> MKKSLGARTLAYPTPLFLVGTYDRDSRPNIMAAAWAGICCSQPPSIAVSLRKATYTYRSITERGAFTISIPSRAYVRHADYAGIYSGENEDKFASLGLTPVPGEHVDAPYVGEFPMAIELKLIHQIEIGLHTQFIGEIMD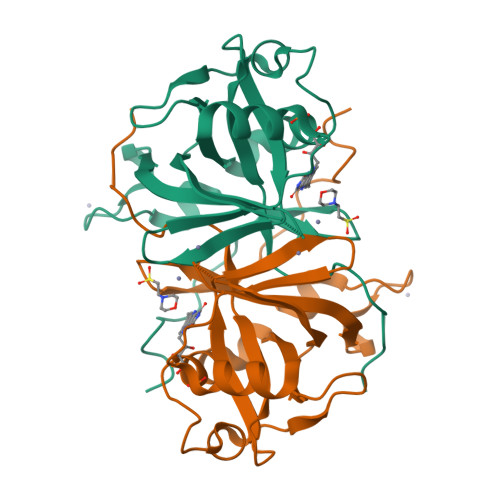VKVDESCLRDDGLPDINKVDPVIFAPVSREYYAVGEFLAKAFSAGKGLRS2,4-DIHYDROXY-N-[2-(2-MERCAPTO-VINYLCARBAMOYL)-ETHYL]-3,3-DIMETHYL-BUTYRAMIDE | C11 H20 N2 O4 S | 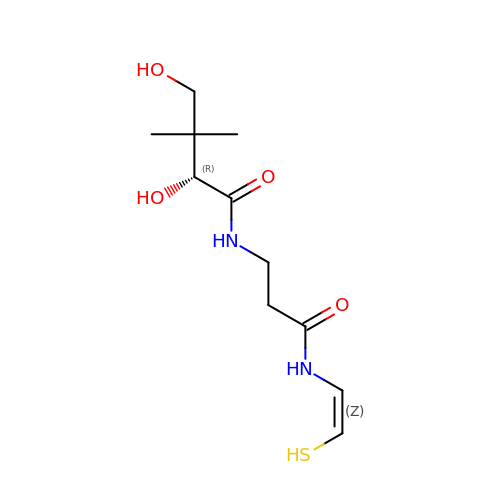GVPONLWGQFZYSV-UDIARPCQSA-N>[2x]GPLGSMGKKSRVKTQKSGTGATATVSPKEILNLTSELLQKCSSPAPGPGKEWEEYVQIRTLVEKIRKKQKGLSVTFDGKREDYFPDLMKWASENGASVEGFEMVNFKEEGFGLRATRDIKAEELFLWVPRKLLMTVESAKNSVLGPLYSQDRILQAMGNIALAFHLLCERASPNSFWQPYIQTLPSEYDTPLYFEEDEVRYLQSTQAIHDVFSQYKNTARQYAYFYKVIQTHPHANKLPLKDSFTYEDYRWAVSSVMTRQNQIPTEDGSRVTLALIPLWDMCNHTNGLITTGYNLEDDRCECVALQDFRAGEQIYIFYGTRSNAEFVIHSGFFFDNNSHDRVKIKLGVSKSDRLYAMKAEVLARAGIPTSSVFALHFTEPPISAQLLAFLRVFCMTEEELKEHLLGDSAIDRIFTLGNSEFPVSWDNEVKLWTFLEDRASLLLKTYKTTIEEDKSVLKNHDLSVRAKMAIKLRLGEKEILEKAVKSAAVNREYYRQQMEEKAPLPKYEESNLGLLESSVGDSRLPLVLRNLEEEAGVQDALNIREAISKAKATENGLVNGENSIPNGTRSENESLNQESKRAVEDAKGSSSDSTAGVKE;>TLKYPIEHGIVTNWD[2x]

Here we elucidate the structural and molecular determinant(s) of target specificity of histidine vs. lysine in the active site of SETD3. On the substrate-binding surface, the residues are diverse, reflecting the fact that the three enzymes act on three very distinct substrates—the large subunit of Rubisco by LSMT, RelA subunit of nuclear factor NFκB by SETD6, and actin by SETD3—with limited sequence similarity immediately surrounding the methylation target. To facilitate the methyl transfer reaction, SETD3 provides a local environment that promotes deprotonation of the target nitrogen N3 of histidine (and concomitant protonation of N1). Most (if not all) SAM-dependent MTases use the classic SN2 reaction mechanism, which requires the target nitrogen be in a deprotonated state.

First, we used the SAM analog sinefungin (adenosyl ornithine) to prepare a complex mimicking the pre-reactive state. Like SAM, sinefungin also carries a formal positive charge, but does not support the methyl transfer, and thus functions as an inhibitor. The target histidine’s imidazole ring is nearly parallel to the aromatic ring of Tyr312, and, to maximize the H-bond potential of both nitrogen atoms, the imidazole ring is positioned such that N3 donates a proton to the main-chain carbonyl oxygen atom of Asp274 (N3–H•••O = C), while the N1 accepts a proton from a water molecule (numbered as w1). This water molecule is coordinated adjacent to the histidine-binding pocket, and is saturated with four H-bonds, three of which are at a traditional H-bond distance from the interacting atoms: the N1 atom of the histidine (2.8 Å), the main-chain carbonyl oxygen atom of Thr252 (2.6 Å) and the side-chain hydroxyl oxygen atom of Ser324 (2.7 Å). The fourth H-bond to w1 is weak and is within a distance of 3.4–3.5 Å from the main-chain carbonyl oxygen of the target histidine, the Cα atom of actin residue G74, or one of the guanidino nitrogen atoms of Arg315. The main difference between the pre-reactive and post-reactive complex structures is that the imidazole ring of methylated His73 rotated away from that of histidine.>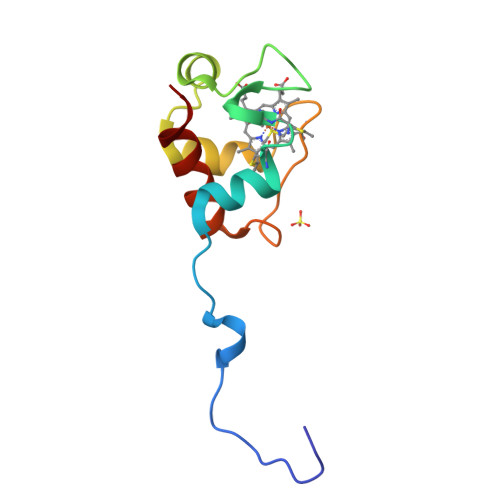 AASWSHPQFEKGAETAVPNSGGGELFATHCAGCHPQGGNTVHPEKTLARARREANGIRTVRDVAAYIRNPGPGMPAFGEAMIPPADALKIGEYVVASFP Influenza virus neuraminidase (NA) is an important target for protective antibodies and therapeutic drugs against influenza viruses. NA cleaves off host sialic acids, aiding the release of newly formed virions from infected cells. NA is a mushroom-shaped type II homotetrameric protein. The polypeptide chain of the NA monomeric head folds into six, topologically identical, four-stranded, antiparallel β-sheets which are arranged like the blades of a propeller.

We found that H5N1 A/mute swan/England/053054/2021 NA (mSN1) expressed at ~380 mg/l as a tetramer with minimal aggregation, exhibiting high enzymatic activity and a high melting temperature. To assess whether loop grafting influenced the local or overall structure of the NA, we determined high resolution crystal structures of mSN1, the N1/09 hybrid, and the N1/19 hybrid. Analysis of mSN1, N1/09 hybrid, and N1/19 hybrid structures revealed some variability in active site conformations, with the greatest variability existing between the cavities of two msN1 molecules within the asymmetric unit of the crystal, reflecting different trajectories of the B1L23 (150-loop). The msN1 structure revealed differences among the protomers of the tetramer at the active site entrance. Within the same tetramer, protomers with a relatively narrow cavity (i) combine with protomers showing a wider entrance (ii). This difference is dictated by the trajectory of the B1L23 loop (150-loop; dark blue with yellow side chains). The variation in trajectory between (i) and (ii) is most pronounced at Val149 (red surface). While the scaffold is structurally conserved across the three resolved structures, each possesses unique active site conformations, which are primarily influenced by the L01 and L23 loops surrounding the active site cavity. All NA proteins were immunogenic in mice, generating binding and NAI antibodies to themselves. mSN1 elicited NAI antibody titres against itself that cross-inhibited viral N1/09 NA. mSN1 showed sufficient cross-reactivity to N1/09 to protect mice against virus challenge.

>[2x]MNTQILVFALIAIIPTNADKISAWSHPQFEKGGGGSHHHHHHSSSGSGAHIVMVDAYKPTKGGSGGGGSIINETADDIVYRLTVIIDDRYESLKNLITLRADRLEMIINDNVSTILAGGSGTGSVTLAGNSSLCPISGWAIYSKDNGIRIGSKGDVFVIREPFISCSHLECRTFFLTQGALLNDKHSNGTVKDRSPYRTLMSCPVGEAPSPYNSRFESVAWSASACHDGISWLTIGISGPDNGAVAVVKYNGIITDTIKSWRNNILRTQESECACVNGSCFTVMTDGPSNGQASYKIFKIEKGKVVKSVELNAPNYHYEECSCYPDAGDIMCVCRDNWHGSNRPWVSFNQNLEYQIGYICSGVFGDNPRPNDGTGSCSPMSSNGAYGVKGFSFKYGNGVWIGRTKSTSSRSGFEMIWDPNGWTETDSSFSVKQDIVEITDWSGYSGSFVQHPEMTGLDCMRPCFWVELIRGRPKENTIWTSGSSISFCGVNSDTVGWSWPDGAELPFTIDK>[3x]VMTMRGLLVGKM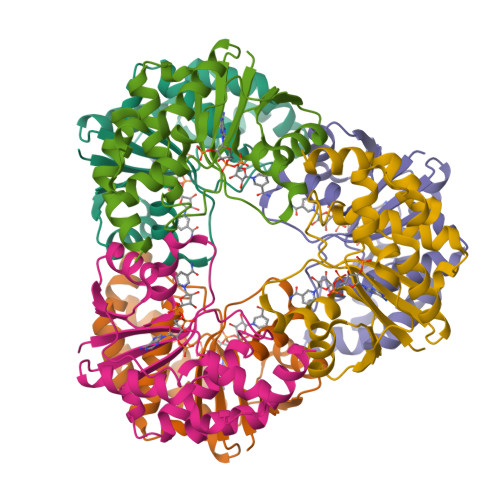QPFHRGHLQVIKSILEEVDELIICIGSAQLSHSIRDPFTAGERVMMLTKALSENGIPASRYYIIPVQDIECNALWVGHIKMLTPPFDRVYSGNPLVQRLFSEDGYEVTAPPLFYRDRYSGTEVRRRMLDDGDWRSLLPESVVEVIDEINGVERIKHLAKKEVSELGGIS(3S,5R,7R,8S,9S,10R)-7-(hydroxymethyl)-3-(4-methylphenyl)-1,6-dioxa-2-azaspiro[4.5]decane-8,9,10-triol 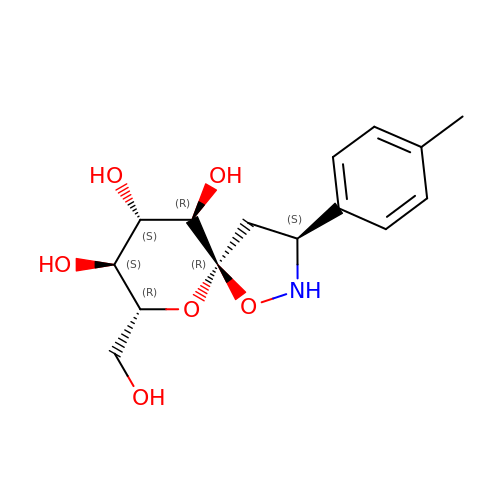| C15 H21 N O6 | HRCKGDOSPBFICB-MZHQWRCYSA-N> QQLYQPFRPPSSPIPTQFR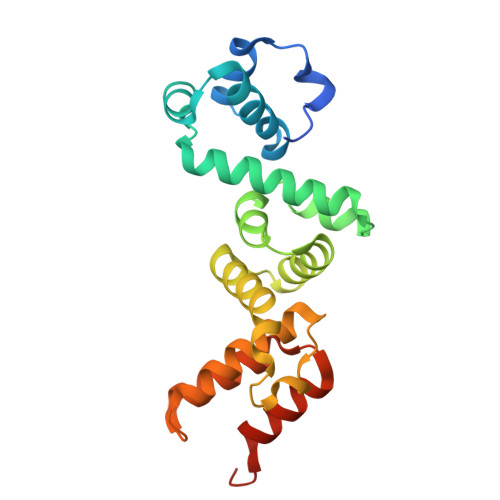SLDSAGKIEILAGRMALWFEYAPLISSLYTDGFTPPTIEELTGISSIEQNRLIVGAQVRDSILQSIHEPELISAFDTGGAELLYEIRLLSTTQRVAAATFIIDRNIDSKGAQDLARAIKDYPNRRGDVGWLDFDYNLPGDCLSFLYYRQSRENKNPSDQRTSMLLQALGVAESEKAKNRLNTELYGDKEAEKEK>MEDLIDGIIFAANYLGSTQLLSDKTPSKNVRMMQAQEAVSRIK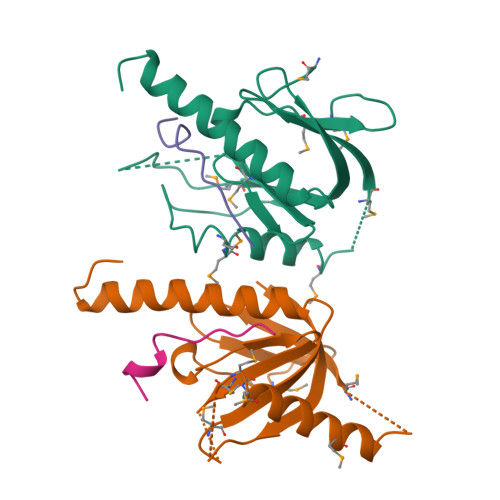MAQKLAKSRKKAPEGESQPMTEVDLFILTQRIKVLNADTQETMMDHPLRTISYIADIGNIVVLMARRRIPRSNSQENVEASHPSQDGKRQYKMICHVFESEDAQLIAQSIGQAFSVAYQEFLRANGINP[2x];>QNGYENPTYKFFE[2x]>GSTGSHTYQHQALVDQLHELIANTDLNKLSYLNLDAFQKRDILAAHYIAKSAIRTKNLDQMTKA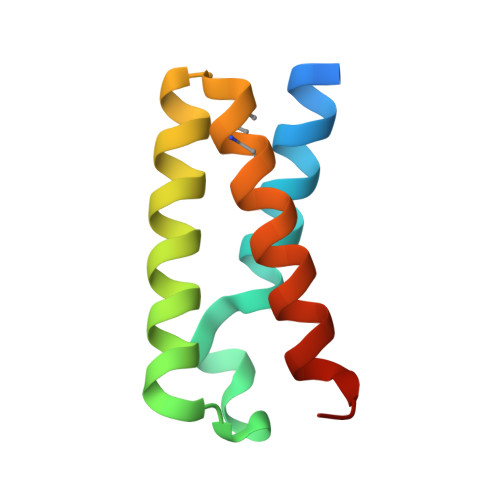KQRLESIYNSISNPLHS[2x]>[2x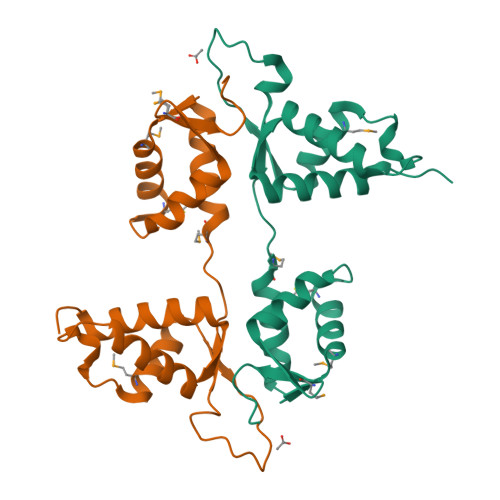]MANEEDDPVVQEIDVYLAKSLAEKLYLFQYPVRPASMTYDDIPHLSAKIKPKQQKVELEMAIDTLNPNYCRSKGEQIALNVDGACADETSTYSSKLMDKQTFCSSQTTSNTSRYAAALYRQGELHLTPLHGILQLRPSFSYLDKADAKHREREAANEAGDSSQDEAEDDVKQITVRFSRPESEQARQRRVQSYEFLQKKHAEEPWVHLHYYGLRDSRSEHERQYLLCPGSSGVENTELVKSPSEYLMMLMPPSQEEEKDKPVAPSNVLSMAQLRTLPLADQIKILMKNVKVMPFANLMSLLGPSIDSVAVLRGIQKVAMLVQGNWVVKSDILYPKDSSSPHSGVPAEVLCRGRDFVMWKFTQSRWVVRKEVATVTKLCAEDVKDFLEHMAVVRINKGWEFILPYDGEFIKKHPDVVQRQHMLWTGIQAKLEKVYNLVKETMPKKPDAQSGPAGLVCGDQRIQVAKTKAQQNHALLERELQRRKEQLRVPAVPPGVRIKEEPVSEEGEEDEEQEAEEEPMDTSPSGLHSKLANGLPLGRAAGTDSFNGHPPQGCAPTPVARELKAFVEATFQRQFVLTLSELKRLFNLHLASLPPGHTLFSGISDRMLQDTVLAAGCKQILVPFPPQTAASPDEQKVFALWESGDMSDQHRQVLLEIFSKNYRVRRNMIQSRLTQECGEDLSKQEVDKVLKDCCVSYGGMWYLKGTVQS>MLGLKTSIIGRRVIYFQEITSTNEFAKTSYLEEGTVIVADKQTMGHGALNRKWESPEGGLWLSIVLSPKVPQKDLPKIVFLGAVGVVETLKEFSIDGRIKWPNDVLVNYKAIAGVLVEGKGDKIVLGIGLNVNNKVPNGATSMKLELG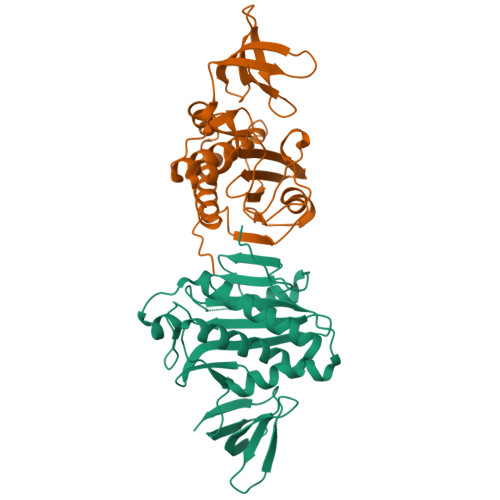SEVPLLSVFRSLITNLDRLYLNFLKNPMDILNLVRDNMILGVRVKILGDGSFEGIAEDIDDFGRLIIRLDSGEVKKVIYGDVSLRFL[2x]> MIVSDIEANALLESVTKFHCGVIYDYSTAEYVSYRPSDFGAYLDALEAEVARGGLIVFHNGHKYDVPALTKLAKLQLNREFHLPRENCIDTLVLSRLIHSNLKDTDMGLLRSGKLPGALEAWGYRLGEMKGEYKDDFKRMLEEQGEEYVDGMEWWNFNEEMMDYNVQDVVVTKALLEKLLSDKHYFPPEIDFTDVGYTTFWSESLEAVDIEHRAAWLLAKQERNGFPFDTKAIEELYVELAARRSELLRKLTETFGSWYQPKGGTEMFCHPRTGKPLPKYPRIKTPKVGGIFKKPKNKAQREGREPCELDTREYVAGAPYTPVEHVVFNPSSRDHIQKKLQEAGWVPTKYTDKGAPVVDDEVLEGVRVDDPEKQAAIDLIKEYLMIQKRIGQSAEGDKAWLRYVAEDGKIHGSVNPNGAVTGRATHAFPNLAQIPGVRSPYGEQCRAAFGAEHHLDGITGKPWVQAGIDASGLELRCLAHFMARFDNGEYAHEILNGDIHTKNQIAAELPTRDNAKTFIYGFLYGAGDEAIGQIVGAGKERGKELKKKFLENTPAIAALRESIQQTLVESSQWVAGEQQVKWKRRWIKGLDGRKVHVRSPHAALNTLLQSAGALICKLWIIKTEEMLVEKGLKHGWDGDFAYMAWVHDEIQVGCRTEEIAQVVIETAQEAMRWVGDHWNF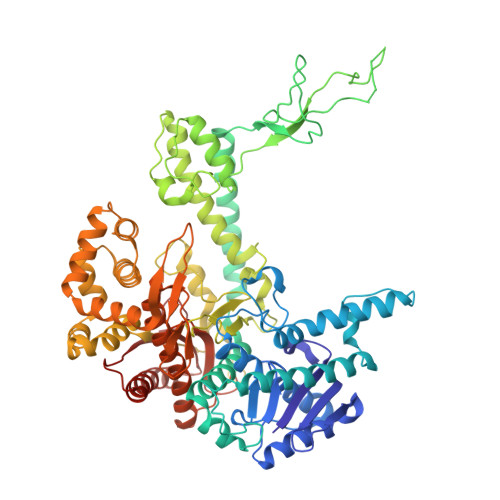RCLLDTEGKMGPNWAICH>[2x]EEIRPKEVYLDRKL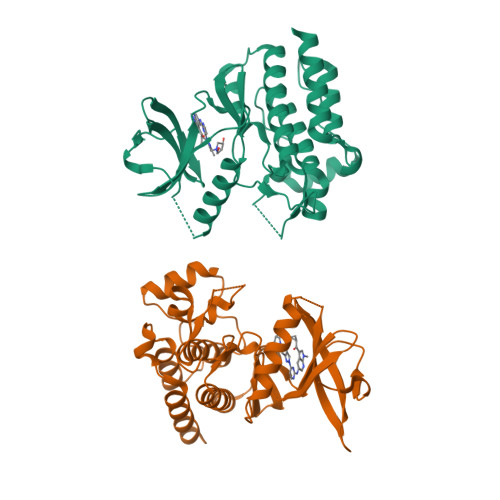LTLEDKELGSGNFGTVKKGYYQMKKVVKTVAVKILKNEANDPALKDELLAEANVMQQLDNPYIVRMIGICEAESWMLVMEMAELGPLNKYLQQNRHVKDKNIIELVHQVSMGMKYLEESNFVHRDLAARNVLLVTQHYAKISDFGLSKALRADENYYKAQTHGKWPVKWYAPECINYYKFSSKSDVWSFGVLMWEAFSYGQKPYRGMKGSEVTAMLEKGERMGCPAGCPREMYDLMNLCWTYDVENRPGFAAVELRLRNYYYDVVNLEHHHHHHHH> SSLDDKPQFPGASAEFIDKLEFIQPNVISGIPIYRVMDRQGQIINPSEDPHLPKEKVLKLYKSMTLLNTMDRILYESQRQGRISFYMTNYGEEGTHVGSAAALDNTDLVFG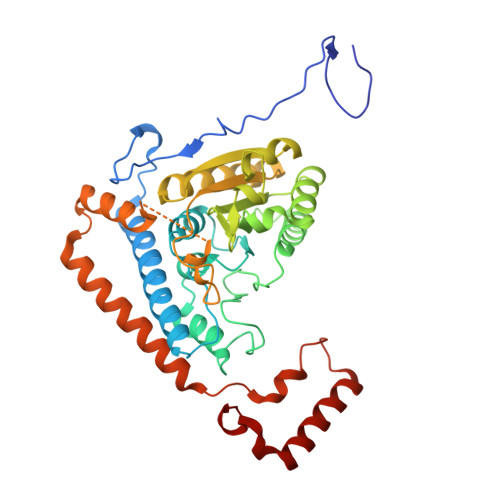QYREAGVLMYRDYPLELFMAQCYGNISDLGKGRQMPVHYGCKERHFVTISSPLATQIPQAVGAAYAAKRANANRVVICYFGEGAASEGDAHAGFNFAATLECPIIFFCRNNGYAISTPTSEQYRGDGIAARGPGYGIMSIRVDGNDVFAVYNATKEARRRAVAENQPFLIEAMTYRIGHHSTSDDSSAYRPVDEVNYWDKQDHPISRLRHYLLSQGWWDEEQEKAWRKQSRRKVMEAFEQAERKPKPNPNLLFSDVYQEMPAQLRKQQESLARHLQTYGEHYPLDHFDK2-amino-5-({[(1S,4S,5R)-4,5-dihydroxycyclopent-2-en-1-yl]amino}methyl)-3,7-dihydro-4H-pyrrolo[2,3-d]pyrimidin-4-one 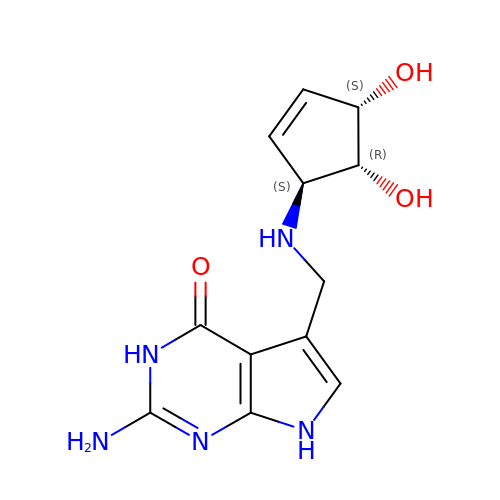| C12 H15 N5 O3 | WYROLENTHWJFLR-ACLDMZEESA-N>MATSGFSKPLHYPPVRRDETVVDDYFGVKVADPYRWLEDPNSEETKEFVDNQEKLANSVLEECELIDKFKQKIIDFVNFPRCGVPFRRANKYFHFYNSGLQAQNVFQMQDDLDGKPEVLYDPNLREGGRSGLSLYSVSEDAKYFAFGIHSGLTEWVTI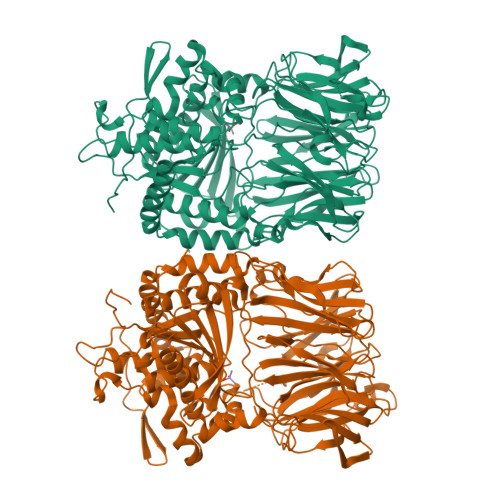KILKTEDRSYLPDTLEWVKFSPAIWTHDNKGFFYCPYPPLKEGEDHMTRSAVNQEARYHFLGTDQSEDILLWRDLENPAHHLKCQITDDGKYFLLYILDGCDDANKVYCLDLTKLPNGLESFRGREDSAPFMKLIDSFDASYTAIANDGSVFTFQTNKDAPRKKLVRVDLNNPSVWTDLVPESKKDLLESAHAVNENQLILRYLSDVKHVLEIRDLESGALQHRLPIDIGSVDGITARRRDSVVFFKFTSILTPGIVYQCDLKNDPTQLKIFRESVVPDFDRSEFEVKQVFVPSKDGTKIPIFIAARKGISLDGSHPCEMHGYGGFGINMMPTFSASRIVFLKHLGGVFCLANIRGGGEYGEEWHKAGFRDKKQNVFDDFISAAEYLISSGYTKARRVAIEGGSNGGLLVAACINQRPDLFGCAEANCGVMDMLRFHKFTLGYLWTGDYGCSDKEEEFKWLIKYSPIHNVRRPWEQPGNEETQYPATMILTADHDDRVVPLHSFKLLATMQHVLCTSLEDSPQKNPIIARIQRKAAHYGRATMTQIAEVADRYGFMAKALEAPWID[2x]> MAAAYKEAFAAVKELMQTSNKPQNVQTAINNTGSKYGKTTVQKALDELVAQNLCIYTEIGKTGKLYLWNQNLLEVLSDAQLMEVNAQINDLKAQVEKLTQQGETLRITQRNLEAAPITEVLKQEVDELRQQVSANDEKLRLVRESNAIVSDADMLTLQKNYKDAMTAWATRRAKCREVIDTLSEGMGVKPSAFMDQLGLEEGLPMTTYTEMKKALPPVNVSKADIKAA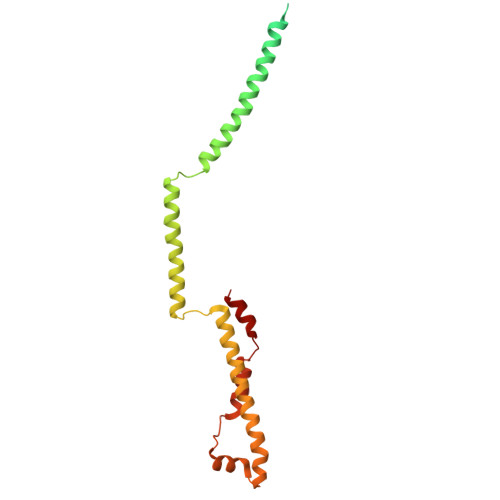LKK> VHVAQTPRSATKESGETLTINCALRDTSYGLHSTAWYRQTPGQSRRDQLTIGGRYVKTVNKPQKTFSLQIRNLVVEDTATYTCRGWVGGREGYEGAGTKLT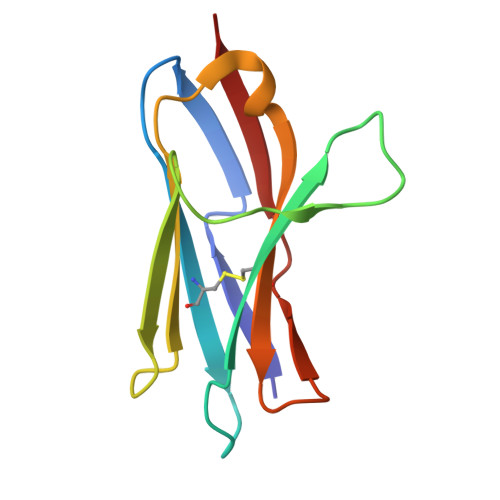VKP> QRDDFHWEEYLKETGSISAPSECFRQSQIPPVNDF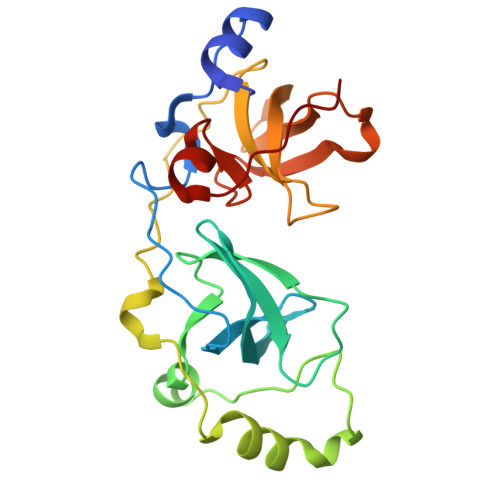KVGMKLEARDPRNATSVCIATVIGITGARLRLRLDGSDNRNDFWRLVDSPDIQPVGTCEKEGDLLQPPLGYQMNTSSWPMFLLETLNGSEMASATLFKKEPPKPPLNNFKVGMKLEAIDKKNPYLICPATIGDVKGDEVHITFDGWSGAFDYWCKYDSRDIFPAGWCRLTGDVLQPPGTS4-[(~{Z})-1-cyano-2-[4-[2-(dimethylamino)ethyl-methyl-amino]phenyl]ethenyl]benzenecarbonitrile 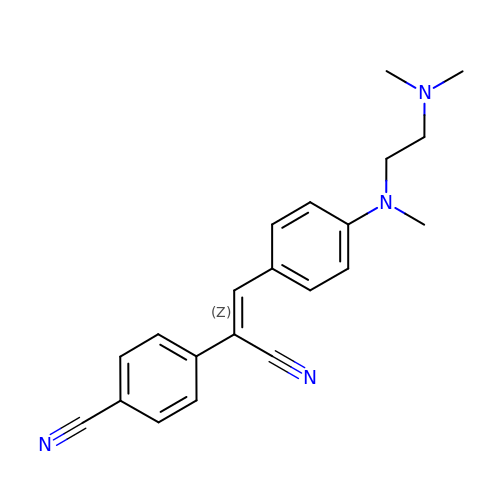| C21 H22 N4 | BCLYGBLOTWSFBR-XSFVSMFZSA-N Francisella virulence arises from a 33 kilobase (Kb) pathogenicity island (FPI) that is regulated by the macrophage locus protein A (MglA) and the stringent starvation protein A (SspA). These proteins interact with both RNA polymerase (RNAP) and the pathogenicity island gene regulator (PigR) to activate FPI transcription. Indeed, while most bacterial SspA proteins function as homodimers to activate transcription, F. tularensis SspA forms a heterodimer with the MglA protein, which is unique to F. tularensis. Thus, our structure unveils MglA as a new member of the SspA subclass of GST proteins.

To gain insight into the function of the F. tularensis MglA protein we determined its structure by multiple wavelength anomalous diffraction (MAD). The crystal contains two molecules of MglA in the asymmetric unit (ASU), which form a dimer. The structure was refined to final Rwork and Rfree values of 17.3% and 22.8%, respectively to 2.95 Å resolution. Each MglA subunit harbors four β strands and 8 α helices. MglA homodimerization is primarily electrostatic and is mediated by 14 salt bridges formed between residues on α4 and α5. Specifically, Arg64, Lys87, Arg89, and Arg93 interact with Asp59', Glu70', Asp74' and Glu97', respectively (where ' indicates the other subunit in the dimer). Indeed, similar to what is observed in SspA proteins, MglA dimerization is largely mediated by contacts between one region from each subunit. This leads to the creation of a V shaped morphology in the MglA dimer, whereby the tightly interacting regions of the dimer combine to create a compact surface (“compact face”) while the opposite side of the dimer harbors a large and exposed cavity (“open face”). Thus, the combined SEC and crosslinking data demonstrate that while MglA appears to preferentially heterodimerize with SspA, it can form weak homodimers in solution. Finally, the MglA structure revealed malate, which was used in crystallization, bound in an open pocket formed by the dimer, suggesting the possibility that this cleft could function in small molecule ligand binding. The relatively low resolution of the structure makes the precise docking of the malate molecules into the density ambiguous and isothermal titration calorimetry experiments revealed no binding suggesting that the observed protein-malate interactions likely occur only at the high malate concentrations (2.1 M) used for crystallization.

>SNAMLLYTKKDDIYSDIVRMILLIKGANAKIVDVSKEENSKHLEELNIITPNGNIPTLSTDDFAVYRLSVIIEAIEDLYPFPPMFPVFPKQRANARILLEYVNKTFLQNIIKLQSPDLDEKQANEIKMLMQRDIISTYKKIVSEREVNAESNPDAQNINVLTLIITFVFYYFIKLKISIPTKDKNIIKEIKELLSEPNFIKTIKAKGA[2x]2-(1-{2-[bis(2-{4-[2-({(6R)-5-(acetylamino)-3,5-dideoxy-6-[(1R,2R)-1,2,3-trihydroxypropyl]-beta-L-threo-hex-2-ulopyranonosyl}oxy)ethyl]-1H-1,2,3-triazol-1-yl}ethyl)amino]ethyl}-1H-1,2,3-triazol-4-yl)ethyl (6R)-5-(acetylamino)-3,5-dideoxy-6-[(1R,2R)-1,2,3-trihydroxypropyl]-beta-L-threo-hex-2-ulopyranosidonic 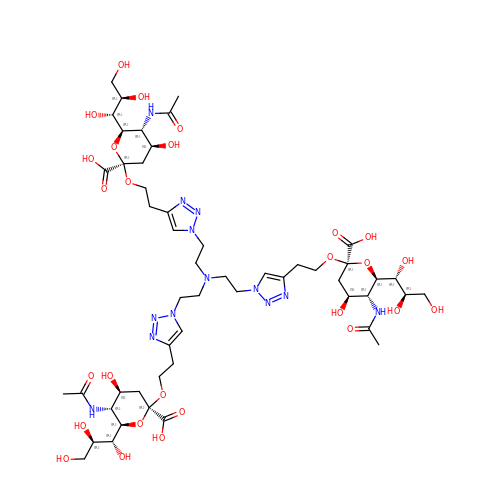acid | C51 H81 N13 O27 | BLJKNJLUKOGWGY-UYSYNVRDSA-N> MGSDKIHHHHHHMHMKTVRQERLKSIVRILERSKEPVSGAQLAEELSVSRQVIVQDIAYLRSLGY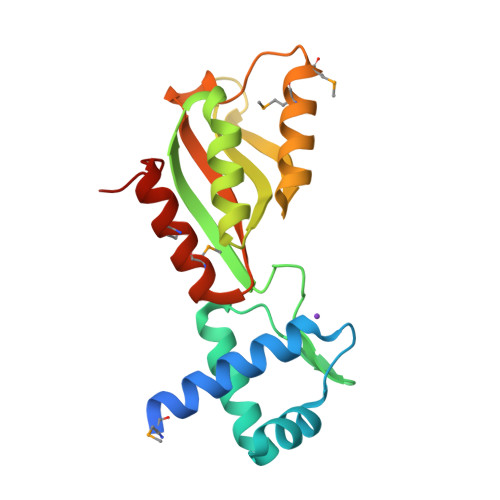NIVATPRGYVLAGGKSGVSRLVAVKHAPEEIKEELLCVVRNGGRIVDVIVEHPVYGEIRGIIDVSSEEEVLKFVNLMEMAKTEPLLTLSGGVHLHTIEAPDEETMERIMRELKKKGFLIEEG> EDSLGMEVGYRLIPMVDFQQDGELLGRIRSIRKKFAQDMGFLPPVVHIRDNMDLQPARYRILMKGVEIGSGDAYPGRWLAINPGTAAGTLPGEKTVDPAFGLDAIWIESALKEQAQIQGFTVVEASTVVATHLNHLIGQFSAELFGRQEAQQLLDRVSQEMPKLTEDLVPGVVTLTTLHKVLQNLLAEKVPIRDMRTILETLAEHAPLQSDPHELTAVVRVALGRAITQQWFPGNEEVQVIGLDTALERLLL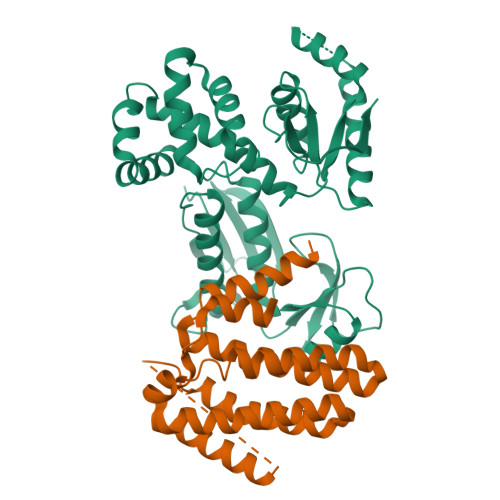QALQGGGGLEPGLADRLLAQTQEALSRQEMLGAPPVLLVNHALRPLLSRFLRRSLPQLVVLSNLELSDNRHIRMTATIG;> MYTASGIKAYAQVSVESAVMSASPHQLIEMLFDGANSALVRARLFLEQGDVVAKGEALSKAINIIDNGLKAGLDQEKGGEIATNLSELYDYMIRRLLQANLRNDAQAIEEVERLLSNIAEAWKQISPKASFQESRGTASGAGGSEGGGSEGGTSGATEDSDYATEVSNMSRAQILQQAGTSVLAQANQVPQNVLSLLR> MAGAQDFVPHTADLAELAAAAGECRGCGLYRDATQAVFGAGGRSARIMMIGEQPGDKEDLAGLPFVGPAGRLLDRALEAADIDRDALYVTNAVKHFKFTRAAGGKRRIKKTPSRTEVVACRPWLIAEMTSVEPDVVVLLGATAAKALLGNDFRVTQHRGEVLHVDDVPGDPALVATVHPSSLLRGPKEERESAFAGLVDDLRVAADVR

UdgX excises uracil from uracil-containing DNA to concurrently form a covalent bond with the resulting AP-DNA. Structurally, UdgX is highly similar to family-4 UDGs (F4-UDGs). However, UdgX is unique in possessing a flexible R-loop (105KRRIH109). Our earlier studies allowed us to propose a reaction mechanism of UdgX, which involves the formation of a covalent bond between H109 of UdgX with the C1′ position of the target deoxyribose sugar concurrently with the uracil excision from this site in DNA.

Substitutions of His109 in MsmUdgX with Ser, Gly, Ala, Gln, Cys and Lys showed the loss of its covalent complex formation with DNA but gained canonical UDG activities. In the reactions of the mutant proteins with ssU9, the entire substrate was converted to product by the H109G mutant, while hardly any substrate was utilized by the H109K mutant. However, H109 substitutions by Gln or Lys, showed poor activity. Further, the overlay of all the structures of UdgX H109 mutants showed that the overall structures are very well conserved with a Cα RMSD of ca 0.2 Å. As anticipated, we note a clear difference in the sizes of the active site cavities in the various mutants. When we arranged the mutants in the order of increasing cavity sizes (left), we noted that the canonical UDG activity of the mutants increased with their increasing cavity sizes to begin with and then with a further increase in the cavity size, the UDG activity declined (right). It suggested that the initial increase in UDG activity (H109K to H109Q to H109G) occurred because of the efficiency with which the water molecule could be localized to make a nucleophilic attack on the C1′ position.>[2x]MHHHHHHSSGRENLYFQGSSESVRVVV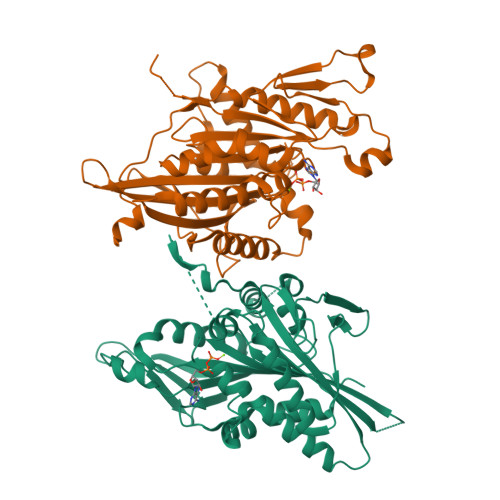RCRPMNGKEKAASYDKVVDVDVKLGQVSVKNPKGTAHEMPKTFTFDAVYDWNAKQFELYDETFRPLVDSVLQGFNGTIFAYGQTGTGKTYTMEGIRGDPEKRGVIPNSFDHIFTHISRSQNQQYLVRASYLEIYQEEIRDLLSKDQTKRLELKERPDTGVYVKDLSSFVTKSVKEIEHVMNVGNQNRSVGATNMNEHSSRSHAIFVITIECSEVGLDGENHIRVGKLNLVDLAGSERQAKTGAQGERLKEATKINLSLSALGNVISALVDGKSTHIPYRDSKLTRLLQDSLGGNAKTVMVANVGPASYNVEETLTTLRYANRAKNIKNKPRVNEDPKDALLREFQ> GNLV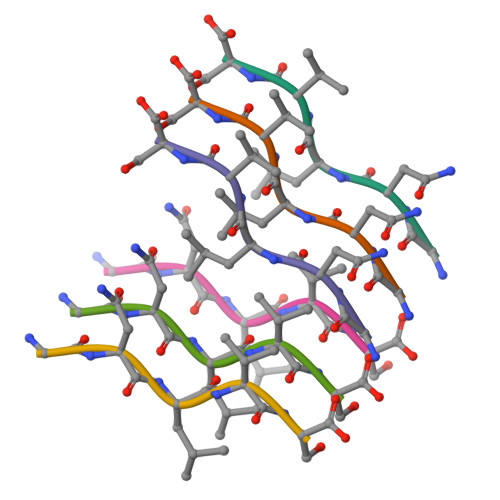S N,N'-bis(2-{(biphenyl-4-ylsulfonyl)[(2R)-1-(hydroxyamino)-3-methyl-1-oxobutan-2-yl]amino}ethyl)benzene-1,3-dicarboxamide (non-preferred 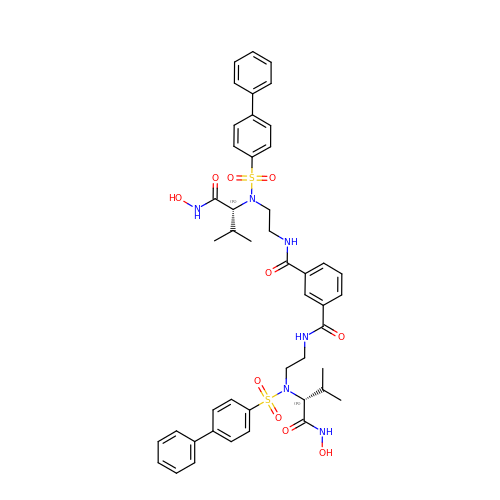name) | C46 H52 N6 O10 S2 | JPMXJRBHCOULJI-NCRNUEESSA-N> QKDANFASGRNSIVHLFEWKWN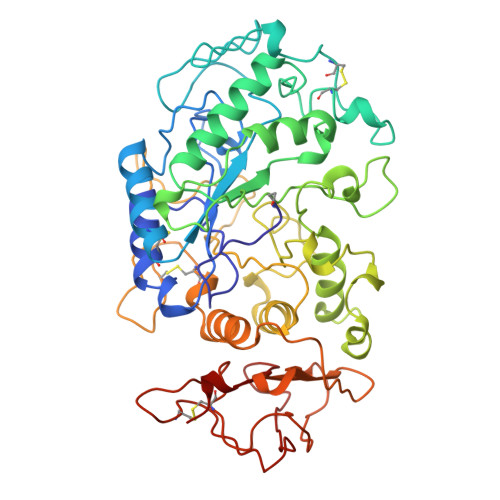DIADECERFLQPQGFGGVQISPPNEYLVADGRPWWERYQPVSYIINTRSGNESAFTDMTRRCNDAGVRIYVDAVINHMTGMNGVGTSGSSADHDGMNYPAVPYGSGDFHSPCEVNNYQDADNVRNCELVGLRDLNAGSDYVRGVLIDYMNHMIDLGVAGFRVDAAKHMSPGDLSVIFDGLKNLNTDYGFADGARPFIYQEVIDLGGEAISKNEYTGFGCVLEFQFGVSLGNAFQGGNQLKNLANWGPEWGLLEGLDAVVFVDNHDNQRTGGSQILTYKNPKPYKMAIAFMLAHPYGTTRIMSSFDFTDNDQGPPQDGSGNLISPGINDDNTCSNGYVCEHRWRQVYGMVGFRNAVEGTQVENWWSNDDNQIAFSRGSQGFVAFTNGGDLNQNLNTGLPAGTYCDVISGELSGGSCTGKSVTVGDNGSADISLGSAEDDGVLAIHVNAKL> ANIVGGIEYSINNASLCSVGFSVTRGATKGFVTAGHCGTVNATARIGGAVVGTFAARVFPGNDRAWVSLTSAQTLLPRVANGSSFVTVRGSTEAAVGAAVCRSGRTTGYQCGTITAKNVTANYAEGAVRGLGQGNACMGRGDSGGSWITSA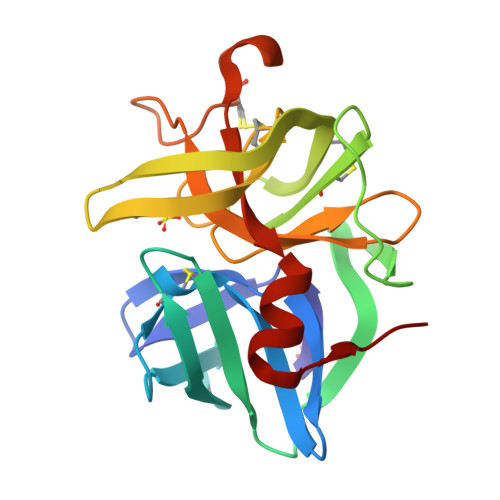GQAQGVMSGGNVQSNGNNCGIPASQRSSLFERLQPILSQYGLSLVTG> ACS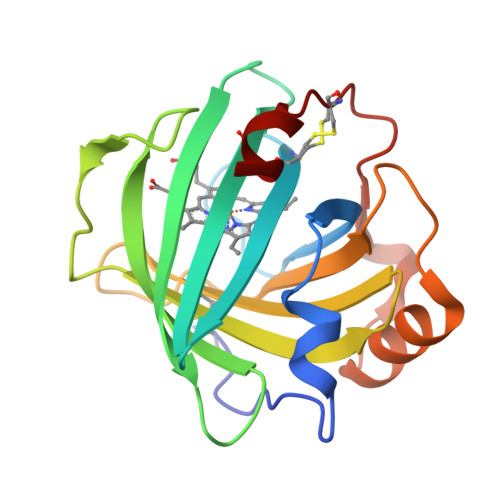TNISPKQGLDKAKYFSGKWYVTHFLDKDPQVTDQYCSSFTPRESDGTVKEALYHYNANKKTSFYNIGEGKLESSGLQYTAKYKTVDKKKAVLKEADEKNSYTLTVLEADDSSALVHICLREGSKDLGDLYTVLTHQKDAEPSAKVKSAVTQAGLQLSQFVGTKDLGCQYDDQFTSL hycanthone | C20 H24 N2 O2 S | 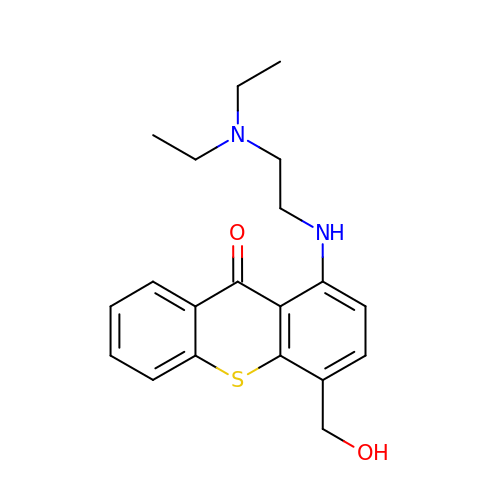MFZWMTSUNYWVBU-UHFFFAOYSA-N>PVVIKTEGPAWTPLEPKLITRLADTVRTKGLRSPITMAEVEALMSSPLLPHDVTNLMRVILGPAPYALWMDAWGVQLQTVIAAATRDPRHPANGQGRGERTNLNRLKGLADGMVGNPQGQAALLRPGELVAITASALQAFREVARLAEPAGPWADIMQGPSESFVDFANRLIKAVEGSDLPPSARAPVIIDCFRQKSQPDIQQLIRTAPSTLTTPGEIIKYVLDRQKTA[3x]

As the virus buds from the cell, the viral protease cleaves Gag into several fragments, including the capsid protein (CA) that then assembles into the mature capsid shell (core), rendering the virus particle infectious. The CA portion of all retroviral Gag proteins folds into two separate domains, the N-terminal domain (CANTD) and C-terminal domain (CACTD). In mature lattices, CANTD interactions form only intra-hexamer and intra-pentamer interfaces, while CACTD interactions are also involved in formation of inter-hexamer and inter-pentamer interfaces. Our results show that, like lentiviruses, RSV is sensitive to IP6 in vitro and in cells, where in the mature CA lattice IP6 binds in a pore formed in the center of the CANTD hexamer.

We acquired cryo-ET data of CASPNC CLPs assembled in the presence of 100 µM IP6. The reconstructed tomograms of this sample showed abundant regular tubes and pleomorphic polyhedral CLPs. Conventional subtomogram averaging of tubular CLPs with regular diameter and shape resulted in a reconstruction of the CA hexamer at 4.3 Å resolution (left). The EM density map revealed a similar arrangement of the CANTD and CACTD, as previously reported for other mature retroviral CLPs. Given the inherent twofold symmetry of the tubes, CA monomers within tubes are present in three symmetry-independent copies. No ordered density for NC and also no ordered density for the β-hairpin, which has been observed in other retroviral mature CAs, were observed. As reported for other mature retrovirus CLPs, intra-hexameric interactions are established via CANTD–CANTD, as well as CANTD–CACTD interfaces, while the inter-hexameric interactions are formed solely via CACTD–CACTD interactions maintaining contacts across twofold and threefold interfaces. Notably, an IP6 molecule could be fitted into the density in the CANTD hexamer center in an upright position, where it is coordinated by two concentric rings of positively charged residues K17 and R21. Hexamers that are separated from pentamers by two or more hexamers, are essentially identical to those found in regular tubes. As the structure of the tube-like hexamer with C2 symmetry was already solved at high resolution from regular tubes, it was not further characterized.>MNRPPATDSGASEFVRSCVNFETNVEFTDVDAYKKTHTAGLASTFVVILGTHAQLREDALKELPFYCPAVAEAIQRVKKGETYAVLAEGVKNEANERFVRVLVGEVPSEASRTNCPARPDVVASLLSAALEEIKGPETKVDVFVRSTAALAIAVAAARSAKRNFTAKEGLATRGYCDN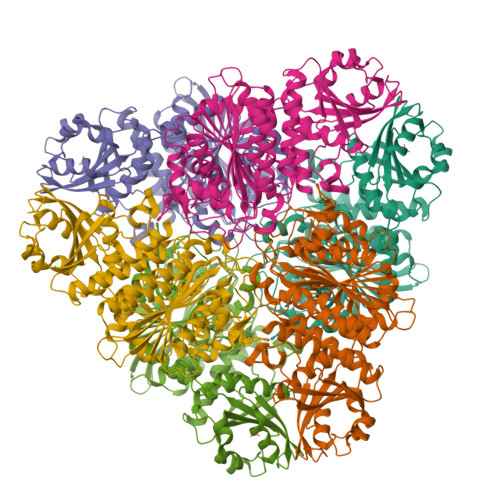CVRLTVVFPTAPNPSPSELAVVATSTQLCQRLVDAPTNLLNTATFAEVAQSYAKELGCAVDVICGEELRERGYGGIYSVGKCAVEAPRLVTLSYKPKDETRKKVALVGKGIVYDSGGLSLKPTNFMTGMKRDMGGAAAVFCGFLTAVRLQMPIELSCTLCLAENAIGPDAYRNDDILTLKSGKTVEVNNTDAEGRLVLGDGVFHATHEISFKPDVLVDMATLTGAQGIATGHRHAGIFVNDEEEELSFLKAGRASGETCFPVLYCPEYHVTEFRSPVADMRNSVKQVNNASVSCAGQFVANHLSPDFKGKHIHVDMAFPAFENDKATGFGPALLTEYLRNLR[2x]The cellulosome is a highly intricate molecular nanomachine produced by anaerobic microorganisms to efficiently deconstruct complex plant cell wall polysaccharides, such as cellulose and hemicellulose. Protein-protein interactions established between dockerin (Doc) modules, located in the cellulosomal enzymes, and cohesin (Coh) modules of the scaffoldin molecule are the primary force for cellulosomal assembly. To date Ruminococcus flavefaciens, a Gram-positive anaerobic bacterium of the Firmicutes phylum, is the only ruminal species that has been shown to assemble a definite cellulosome. Finally, ScaA Doc, the unique member of group 5, binds exclusively to ScaB Cohs 5–9. This latter interaction has a central role in cellulosomal assembly as it allows the binding of up to five ScaA primary scaffoldins to ScaB and up to 10 more enzymes to a single cellulosome.

Here, we report the crystal structure of the R. flavefaciens strain FD-1 Coh-Doc complex established between ScaA Doc and the fifth cohesin of ScaB (RfCohScaB-DocScaA). The structure included two molecules of the RfCohScaB5-DocScaA heterodimer in the asymmetric unit, with each Doc coordinating two calcium (Ca2+) ions, as well as 1 acetonitrile and 225 water molecules. RfCohScaB5 displays an overall typical elliptical Coh structure containing nine β-strands forming two β-sheets in an elongated β-barrel displaying a classical “jelly-roll fold”. β-strands 9, 1, 2, 7, 4 comprise one sheet while β-strands 8, 3, 6, 5 are positioned on the opposite face. RfDocScaA comprises three α-helices, two of which (helix 1: Val-662 to Asp-677; helix 3: Lys-710 to Leu-723) are arranged in an antiparallel orientation forming a planar surface on the Doc that interacts with CohScaB5. These two helices comprise portions of the two classic Doc repeating segments, each containing a bound Ca2+ ion in loops located at opposite ends of the module. In contrast, the pattern of Ca2+ coordination in the C-terminal repeat is displaced due to the 12-residue loop insertion between Pro-693 and Ser-704. Thus, the C-terminal Ca2+ coordination adopts a tetrahedral configuration involving the side chains of residues Asp-689 and Asp-712 (both the Oδ1 and Oδ2) and completed by the main-chain carbonyl groups of Phe-691 and Asp-707. Helices 1 and 3 of RfDocScaA make numerous contacts with RfCohScaB5 β-sheets 8–3–6–5. The side chains of Val-662 and Val-666 at positions 11 and 15 dominate the hydrophobic recognition by contacting with the RfCohScaB5 hydrophobic platform formed by Ala-775/777 and Phe812/852.

>TPATGSAEWVIPTVNAKPGEKVTMDVVVKNSAIEVAGAQFNIKQTAPIAYGSAASGDAYAAIVPNETEQYYAFGEGIGKGIKAADGAKIITLTFNVPADCAKGTYPVKWSNAFITDTNGNKITDKITLTDGAIVVGDT[2x];>[2x]HMASKPVWGDVNCDGDVNVADVVLLNKWLNNNADYAMTDQGKVNADCFNPQDANGGAVDASKVDLTKTDSDAIIKSVVHLITLPAKG Neisseria meningitidis encodes two MarR-family repressors, NMB1853, a homologue of FarR found in N. gonorrhoeae which presumably also controls expression of the FarRAB efflux pump, and a second MarR, NMB1585, of unknown function. The proteins are homodimers comprising a largely helical dimerization domain linked to a DNA-binding domain that contains a winged helix–turn–helix motif. MarR proteins repress the activity of their target genes by binding as dimers to pseudopalindromic sequences in the −10 region of the regulated promoters. The repressor activity of MarR proteins is modulated by co-inducer binding, or in the case of OhrR oxidation of cysteines disrupting disulfide-bridge formation, both of which lead to a major rearrangement in the dimerization region such that the spacing of the DNA-binding domains is significantly altered, preventing DNA recognition.

The structure of NMB1585 was solved to a resolution of 2.1 Å by the multiple-wavelength anomalous dispersion method using seleno­methionine-substituted protein. Overall, the dimeric structure resembles those of other MarR proteins, with each subunit comprising a winged helix–turn–helix (wHtH) domain connected to an α-helical dimerization domain. The dimer interface is thus formed by a symmetrical interaction of the arm domains of the two monomers and involves contacts between both N-terminal and C-­terminal regions (approximately residues 1–25 and 110–142). The spacing of the recognition helices of the wHtH domain indicates that NMB1585 is pre-configured for DNA binding, with a putative inducer pocket that is largely occluded by the side chains of two aromatic residues (Tyr29 and Trp53). Thus, NMB1585 appears to be pre-configured for DNA binding, similar to the structures reported for the HucR regulator of D. radiodurans and a MarR-family protein from S. tokodaii. The residues in the recognition helix (α4) that are most likely to be involved in binding in the major groove of DNA are Gln58, Thr59 and Ser61. Overlaying of NMB1585 and MTH313 confirms the presence of a potential ligand-binding pocket in NMB1585 at a similar location to those in MTH313 and other MarR proteins. Therefore, in order for a ligand to bind into the binding pocket of NMB1585 a conformational change would have to occur in the protein so that the dimerization domain moved away from the DNA-binding domain. Interestingly, the addition of salicylate, a prototypical MarR ligand, did not affect the formation of the protein–DNA complexes, suggesting that the protein does not interact with salicylate, in contrast to E. coli MarR and MTH313. This may be explained by the occluded nature of the putative binding site observed in the crystal structure of NMB1585 and suggests that the protein may adopt this conformation in solution.

>[2x]GPMNQLDQLGTRINLICNVFDKWIGQQDLNYNLFAVLYTLATEGSRTQKHIGEKWSLPKQTVSGVCKTLAGQGLIEWQEGEQDRRKRLLSLTETGKAYAAPLTESAQEFSDKVFATFGDKRTTRLFADLDALAEVMEKTISENKK>[2x]EFVKV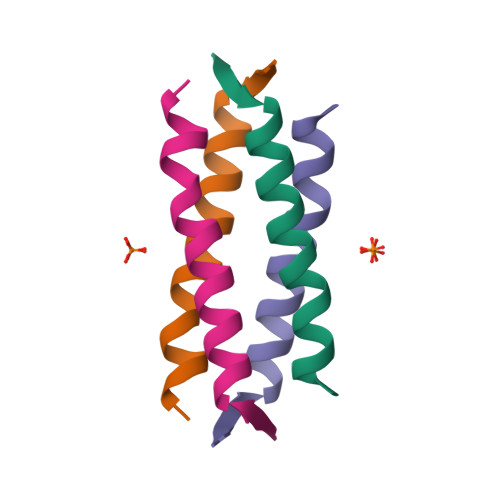RKKDLERLTTEVMQIRDFLPRILNGEV>MAHHHHHHMTHHALIEAAKAAREKAYAPYSNFKVGAALVTNDGKVFHGCNVENASYGLCNCAERTALFSALAAGYRPGEFAAIAVVGETHGPIAPCGACRQVMIELGKPTLEVVLTNMQGDVRVTSAGDL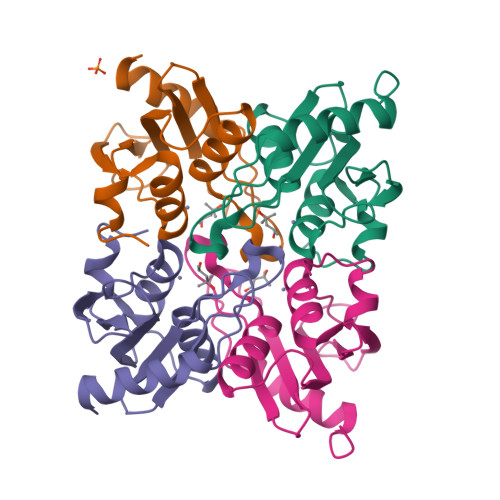LPDAFYLA[4x]> SMNFYSAYQHGFVRVAACTHHTTIGDPAANAASVLDMARACHDDGAALAVFPELTLSGYSIEDVLLQDSLLDAVED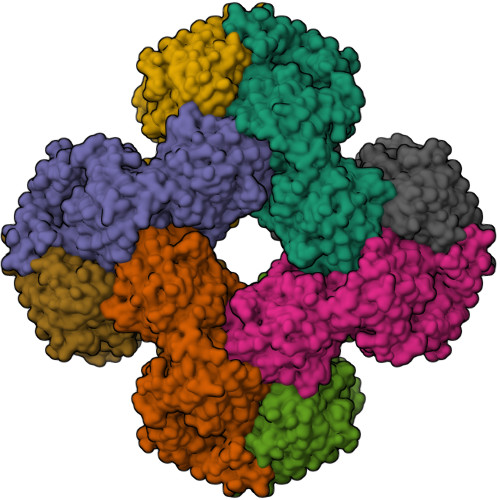ALLDLVTESADLLPVLVVGAPLRHRHRIYNTAVVIHRGAVLGVVPKSYLPTYREFYERRQMAPGDGERGTIRIGGADVAFGTDLLFAASDLPGFVLHVEIAEDMFVPMPPSAEAALAGATVLANLSGSPITIGRAEDRRLLARSASARCLAAYVYAAAGEGESTTDLAWDGQTMIWENGALLAESERFPKGVRRSVADVDTELLRSERLRMGTFDDNRRHHRELTESFRRIDFALDPPAGDIGLLREVERFPFVPADPQRLQQDCYEAYNIQVSGLEQRLRALDYPKVVIGVSGGLDSTHALIVATHAMDREGRPRSDILAFALPGFATGEHTKNNAIKLARALGVTFSEIDIGDTARLMLHTIGHPYSVGEKVYDVTFENVQAGLRTDYLFRIANQRGGIVLGTGDLSELALGWSTYGVGDQMSHYNVNAGVPKTLIQHLIRWVISAGEFGEKVGEVLQSVLDTEITPELIPTGEEELQSSEAKVGPFALQDFSLFQVLRYGFRPSKIAFLAWHAWNDAERGNWPPGFPKSERPSYSLAEIRHWLQIFVQRFYSFSQFKRSALPNGPKVSHGGALSPRGDWRAPSDMSARIWLDQIDREVPKG dihydrostreptomycin | C21 H41 N7 O12 | 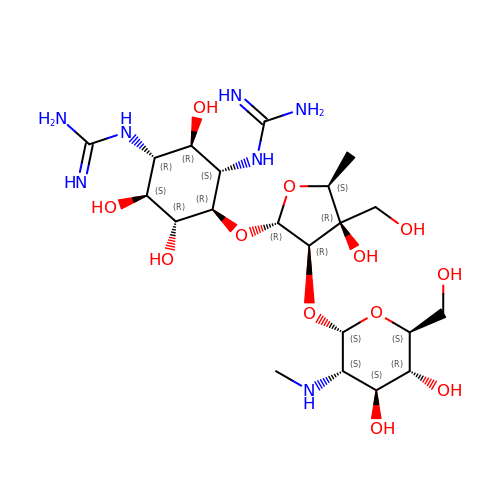ASXBYYWOLISCLQ-HZYVHMACSA-N> MRNEMHLQFSARSENESFARVTVAAFVAQLDPTMDELTEIKTVVSEAVTNAIIHGYNNDPNGIVSISVIIEDGVVHLTVRDEGVGIPDI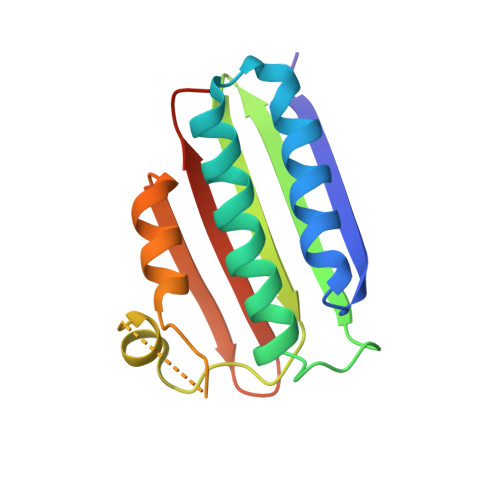EEARQPLFTTKPELERSGMGFTIMENFMDEVIVESEVNKGTTVYLKKHGIHHHHHH> MGSSHHHHHHSSGDDDDKSKSPLRVAVIGGGIAGTALALGLSKSSHVNVKLFETAPAFGEIGAGVSFGVNAVEAIQRLGIGELYKSVADSTPAPWQDIWFEWRHAHDASLVGATVAPGIGQSSIHRAD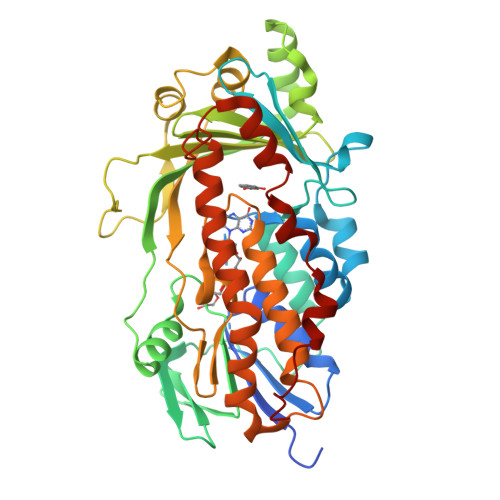FIDMLEKRLPAGIASLGKHVVDYTENAEGVTLNFADGSTYTADVAIAADGIKSSMRNTLLRAAGHDAVHPQFTGTSAYRGLVETSALREAYQAASLDEHLLNVPQMYLIEDGHVLTFPVKKGKLIIIVAFVSDRSVAKPQWPSDQPWVRPATTDEMLHRFAGAGEAVKTLLTSIKSPTLWALHDFDPLPTYVHGRVALIGDAAHAMLPHQGAGAGQGLEDAYFMAELLGNPLHEASDIPALLEVYDDVRRGRASKVQLTSREAGELYEYRTPGVERDTAKLKALLESRMNWIWNYDLGAEARLAVKPALA>MEENGMKSKILIFGGTGYIGNHMVKGSLKLGHPTYVFTRPNSSKTTLLDEFQSLGAIIVKGELDEHEKLVELMKKVDVVISALAFPQILDQFKILEAIKVAGNIKRFLPSDFGVEEDRINALPPFEALIERKRMIRRAIEEANIPYTYVSANCFASYFINYLLRPYDPKDEITVYGTGEAKFAMNYEQDIGLYTIKVATDPRALNRVVIYRPSTNIITQLELISRWEKKIGKKFKKIHVPEEEIVALTKELPEPENIPIAILHCLFIDGATMSYDFKENDVEASTLYPELKFTTIDELLDIFVH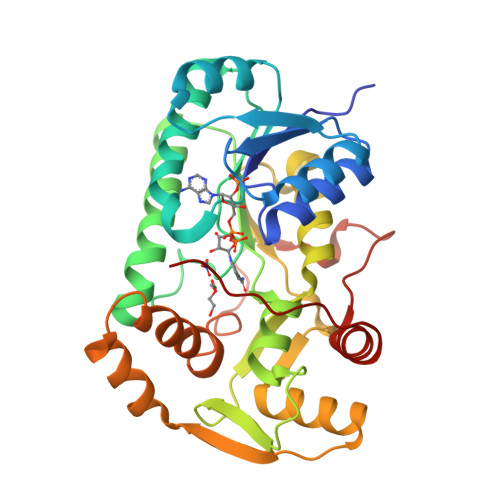DPPPPASAAF[2x]> CTCGA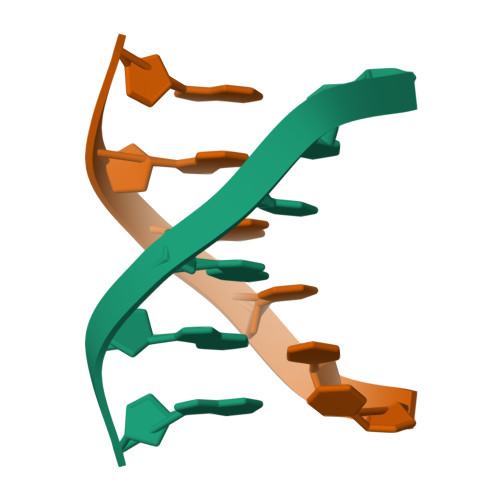G>MQSARMTPSVGRQLLRLGARSSRSTTVLQGQPRPISAQRLYAREATQAVLDKPETLSSDASTREKPARAESKSFAVGMFKGQLTIDQVFPYPSVLSEEQAQFLKELVGPVARFFEEVNDPAKNDALEKVEDDTLQGLKELGAFGLQVPSELGGLGLSNTQYARLAEIVGMHDLGVSVTLGAHQSIGFKGILLYGTKAQREKYLPRVASGQALAAFCLTEPSSGSDVASIRSSAIPSPCGKYYTLNGSKIWISNGGLADIFTVFAKTPIKDAATGAVKEKITAFVVERSFGGVTHGLPEKKMGIKASNTSEVYFDGVKVPSENVLGEVGDGFKVAVNILNNGRFGMAATLAGTMKSLIAKAVDHATNRTQFGDKIHNFGVIQEKLARMAILQYVTESMAYMLSANMDQGFKDFQIEAAISKIFCSEAAWKVADECIQIMGGMGFMKEPGVERVLRDIRIFRIFEGANDILRLFVALQGCMDKGKELTGLGNALKNPFGNVGLLMGEAGKQLRRRTGIGSGLSLSGIVHPELSRSGELAVQALDQFATVVEAKLVKHKKGIVNEQFLLQRLADGAIDLYAMVVVLSRASRSLSEGYPTAQHEKMLCDSWCIEAATRIRENMASLQSSPQHQELFRNFRSISKAMVENGGLVTGNPLGI[2x]

Mammalian complex I (NADH:ubiquinone oxidoreductase) is central to cellular metabolism, with key roles in NAD+ homeostasis, respiration, and oxidative phosphorylation. It couples NADH oxidation in the mitochondrial matrix to ubiquinone reduction in the inner membrane, reoxidizing the NAD+ pool to sustain metabolism, and captures the energy from the redox reaction to transfer protons across the inner membrane and create the proton-motive force that drives ATP synthesis. Complex I is a ‘boot-shaped’ enzyme, with a hydrophilic domain in the mitochondrial matrix that contains the cofactors for redox catalysis, and a membrane-bound domain that transports the protons. Here, we use a popular complex I-linked mitochondrial disease model, the ndufs4−/− mouse, to define the structural, biochemical, and functional consequences of the absence of subunit NDUFS4.

The 12% of particles in ndufs4−/− class 1 were found to have an additional large low-resolution density on the heel of the complex. Particle subtraction of this region followed by local refinement with C2 symmetry produced a 4.2-Å resolution map for the additional density, which was visually identified as a dimer of an ACAD-family protein. Mass spectrometry on purified heart ndufs4−/− complex I (prepared without cross-linking) identified two candidates, ACAD9 and ACADVL, both with mass ~65 kDa (Fig. EV3). Although our complexome analyses of DDM-solubilized ndufs4−/− heart membranes (Figs. 2B and EV1) revealed co-migration of ACAD9 and the ~800 kDa QP subcomplex (but not co-migration of ACADVL), our MALDI-TOF and LC/MS analyses both contained substantially more peptides for ACADVL. Considering the sequence similarity between the two proteins, these data suggest ACADVL is present in greater abundance than ACAD9. We thus chose to model the density as a dimer of ACADVL, and a survey of positions where bulky residues (Tyr, Trp, and Phe) vary between the two subsequently confirmed it as the major species. The resolution achieved was sufficient to model the two FAD cofactors in the ACAD dimer, accounting for the ~0.3 FAD per MDa protein observed in the purified complex (two FAD per dimer bound to 12% of particles). The location of ACAD binding in our map is surprising: ACAD proteins are known to be membrane-associated and located in the mitochondrial matrix, but in our structure the ACAD dimer appears to have ‘slipped’ around, into a position that would be occupied by the lipid tails of a membrane bilayer. Therefore, we conclude the ACAD dimer is artefactually bound, and that its observed binding mode is not physiologically relevant or involved in enzyme assembly.> ATDAASLVGELQAADAEYQNLANQEEARFNEERAQADAARQALAQNEQVYNELSQRA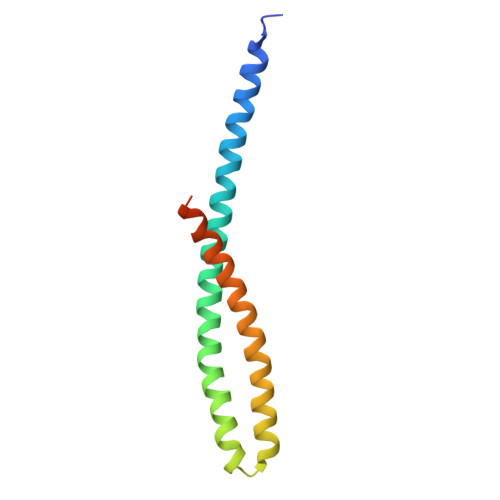QRLQAEANTRFYKSQYQELASKYEDALKKLEAEMEQQKAVISDFEKIQALRAGNLEHHHHHH>[2x]SMDRRRFIKGSMAMAAVCGTSGIASLFSQAAFAADSDIADGQTQRFDFSILQSMAHDLAQTAWRGAPRPLPDTLATMTPQAYNSIQYDAEKSLWHNVENRQLDAQFFHMGMGFRRRVRMFSVDPATHLAREIHFRPELFKYNDAGVDTKQLEGQSDLGFAGFRVFKAPELARRDVVSFLGASYFRAVDDTYQYGLSARGLAIDTYTDSKEEFPDFTAFWFDTVKPGATTFTVYALLDSASITGAYKFTIHCEKSQVI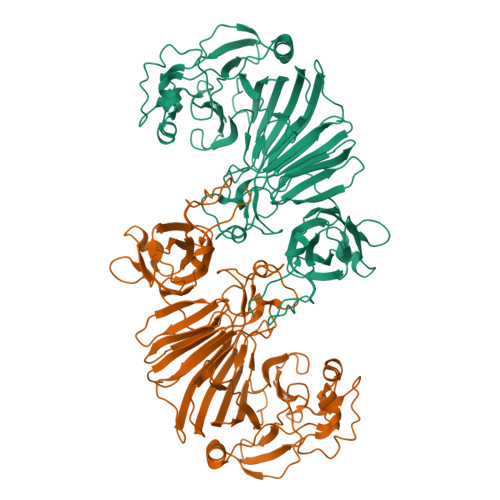MDVENHLYARKDIKQLGIAPMTSMFSCGTNERRMCDTIHPQIHDSDRLSMWRGNGEWICRPLNNPQKLQFNAYTDNNPKGFGLLQLDRDFSHYQDIMGWYNKRPSLWVEPRNKWGKGTIGLMEIPTTGETLDNIVCFWQPEKAVKAGDEFAFQYRLYWSAQPPVHCPLARVMATRTGMGGFSEGWAPGEHYPEKWARRFAVDFVGGDLKAAAPKGIEPVITLSSGEAKQIEILYIEPIDGYRIQFDWYPTSDSTDPVDMRMYLRCQGDAISETWLYQYFPPAPDKRQYVDDRVMS The virulence of P. gingivalis is dependent on secreted cysteine proteases called gingipains (RgpA, RgpB, and Kgp) that are essential for corruption of the host immune system and acquisition of nutrients and heme – a vital growth factor and source of black pigmentation of colonies on blood agar. Gingipains are synthesized with a typical N-terminal signal peptide targeting them to the Sec translocon and are exported through the OM via a novel secretion system referred to as “Por Secretion System; PorSS” or following the naming convention, Type IX Secretion System (T9SS)7. Translocation of gingipains from the periplasm across the OM is dependent on a conserved C-terminal domain (CTD), which appears to be important for secretion of the proteins and in particular, truncation of the last few C-terminal residues of this domain leads to accumulation of gingipains in the periplasm. Here, we show for the first time that the OM translocation signal, a conserved CTD of RgpB, has a typical Ig-like fold encompassing seven antiparallel β-strands organized in two β-sheets that are packed against each other in a β-sandwich.

However, diffraction quality crystals were obtained using mutants of the same construct, which included an inserted hexahistidine after residues S664 or I665 (recombinant products r664i6H and r665i6H, respectively), or by substitution of six consecutive linker residues (I665ADVAN670) with a factor Xa cleavage motif (IEGRAA; r665sXa). The three structures were solved and refined with diffraction data to 1.9 Å, 2.4 Å, and 2.1 Å resolution, respectively. Each variant of rIgSF-CTD formed nearly identical crystal structures (RMSD of 0.760 Å for r665i6H and 0.327 Å for r665sXa, with respect to r664i6H for 298 aligned residues). Thus, we performed our analysis with the structure refined to highest resolution (r664i6H). In each tandem, the IgSF and CTD domains showed an orthogonal arrangement, with their longest axes tilted by 90 degrees with respect to each other. Regions with defined electron density included the residues V579-G662 (IgSF) and K672–K736 (CTD). The 9-residue linker (T663-D671) between the immunoglobulin-like subdomain and the CTD did not yield visible electron density, indicating that this fragment was disordered in the crystals. The hexahistidine tag was inserted in this disordered area. The overall fold of the rCTD distantly resembles that of the IgSF domain, and both domains superimpose with an RMSD of 2.11 Å for 63 aligned residues, despite sharing a sequence identity below 20%.

>[2x]GPTLVPTKMQVTAPANISASAQTFEVACDYNGAIATLSDDGDMVGTAIVKDGKAIIKLNESIADETNLTLTVVGYNKVTVIKDVKVEGTSHHHHHHIADVANDKPYTVAVSGKTITVESPAAGLTIFDMNGRRVATAKNRMVFEAQNGVYAVRIATEGKTYTEKVIVK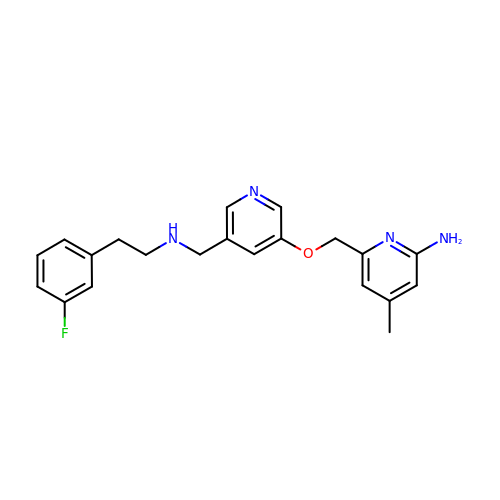6-({[5-({[2-(3-fluorophenyl)ethyl]amino}methyl)pyridin-3-yl]oxy}methyl)-4-methylpyridin-2-amine | C21 H23 F N4 O | IGLNPZZNPBQOMM-UHFFFAOYSA-N>SDELYRQSLEIISRYLREQATGAKDTKPMGRSGATSRKALETLRRVGDGVQRNHETAFQGMLRKLDIKNEDDVKSLSR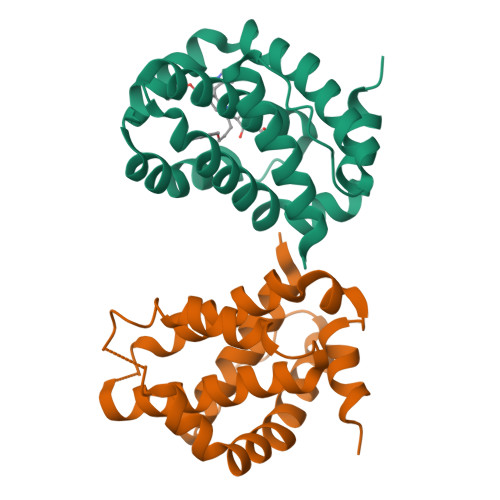VMIHVFSDGVTNWGRIVTLISFGAFVAKHLKTINQESCIEPLAESITDVLVRTKRDWLVKQRGWDGFVEFFHV[2x]> DEGKITVFAAASLTNAMQDIATQFKKEKGVDVVSSFASSSTLARQIEAGAPADLFISADQKWMDYAVDKKAIDTATRQTLLGNSLVVVAPKASVQKDFTIDSKTNWTSLLNGGRLAVGDPEHVPAGIYAKEALQ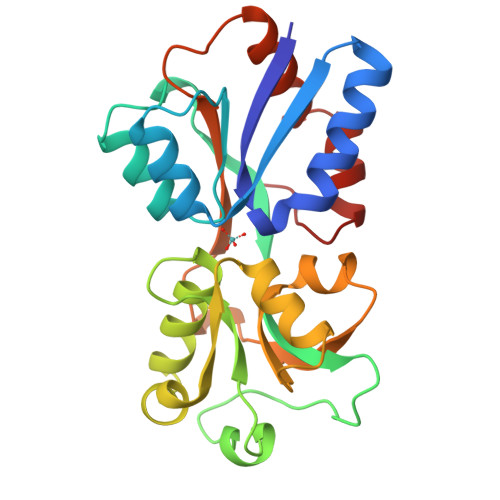KLGAWDTLSPKLAPAEDVRGALALVERNEAPLGIVYGSDAVASKGVKVVATFPEDSHKKVEYPVAVVEGHNNATVKAFYDYLKGPQAAEIFKRYGFTIK>MALALWVFGLLDLICLASANIFEYQVDAQPLRPCELQRERAFLKREDYVPQCAEDGSFQTVQCGKDGASCWCVDADGREVPGSRQPGRPAACLSFCQLQKQQILLSSYINSTATSYLPQCQDSGDYSPVQCDLRRRQCWCVDAEGMEVYGTRQQGRPARCPRSCEIRNRRLLHGVGDRSPPQCSPDGAFRPVQCKFVNTTDMMIFDLVHSYSRFPDAFVTFSSFRSRFPEVSGYCYCADSQGRELAETGLELLLDEIYDTIFAGLDLASTFAETTLYRILQRRFLAVQLVISGRFRCPTKCEVERFAATSFRHPYVPSCHPDGEYQAAQCQQGGPCWCVDSRGQEIPGTRQRGEPPSCAEDQSCPSERRRAFSRLRFGPSGYFSRRSLLLAPEEGPVSQRFARFTASCPPSIKELFLDSGIFQPMLQGRDTRFVAPESLKEAIRGLFPSRELARLALQFTTNAKRLQQNLFGGRFLVKVGQFNLSGALGTRGTFNFSHFFQQLGLPGFQDGRALADLAKPLSVGLNSNPASEAPKASKIDVALRKPVVGSFGFEVNLQENQNALQFLSSFLELPEFLLFLQHAISVPEDIARDLGDVMEMVFSSQGCGQAPGSLFVPACTAEGSYEEVQCFAGDCWCVDAQGRELAGSRVRGGRPRCPTECEKQRARMQSLLGSQPAGSSLFVPACTSKGNFLPVQCFNSECYCVDTEGQPIPGTRSALGEPKKCPSPCQLQAERAFLGTVRTLVSNPSTLPALSSIYIPQCSASGQWSPVQCDGPPEQAFEWYERWEAQNSAGQALTPAELLMKIMSYREAASRNFRLFIQNLYEAGQQGIFPGLARYSSFQDVPVSVLEGNQTQPGGNVFLEPYLFWQILNGQLDRYPGPYSDFSAPLAHFDLRSCWCVDEAGQKLEGTRNEPNKVPACPGSCEEVKLRVLQFIREAEEIVTYSNSSRFPLGESFLAAKGIRLTDEELAFPPLSPSRETFLEKFLSGSDYAIRLAAQSTFDFYQRRLVTLAESPRAPSPVWSSAYLPQCDAFGGWEPVQCHAATGHCWCVDGKGEYVPTSLTARSRQIPQCPTSCERLRASGLLSSWKQAGVQAEPSPKDLFIPTCLETGEFARLQASEAGTWCVDPASGEGVPPGTNSSAQCPSLCEVLQSGVPSRRTSPGYSPACRAEDGGFSPVQCDPAQGSCWCVLGSGEEVPGTRVAGSQPACESPQCPLPFSVADVAGGAILCERASGLGAAAGQRCQLRCSQGYRSAFPPEPLLCSVQRRRWESRPPQPRACQRPQFWQTLQTQAQFQLLLPLGKVCSADYSGLLLAFQVFLLDELTARGFCQIQVKTAGTPVSIPVCDDSSVKVECLSRERLGVNITWKLQLVDAPPASLPDLQDVEEALAGKYLAGRFADLIQSGTFQLHLDSKTFSADTSIRFLQGDRFGTSPRTQFGCLEGFGRVVAASDASQDALGCVKCPEGSYFQDEQCIPCPAGFYQEQAGSLACVPCPEGRTTVYAGAFSQTHCVTDCQKNEVGLQCDQDSQYRASQRDRTSGKAFCVDGEGRRLPWTEAEAPLVDAQCLVMRKFEKLPESKVIFSADVAVMVRSEVPGSESSLMQCLADCALDEACGF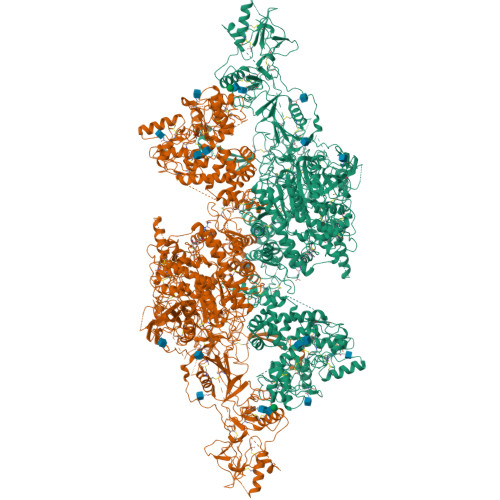LTVSTAGSEVSCDFYAWASDSIACTTSGRSEDALGTSQATSFGSLQCQVKVRSREGDPLAVYLKKGQEFTITGQKRFEQTGFQSALSGMYSPVTFSASGASLAEVHLFCLLACDHDSCCDGFILVQVQGGPLLCGLLSSPDVLLCHVRDWRDPAEAQANASCPGVTYDQDSRQVTLRLGGQEIRGLTPLEGTQDTLTSFQQVYLWKDSDMGSRSESMGCRRDTEPRPASPSETDLTTGLFSPVDLIQVIVDGNVSLPSQQHWLFKHLFSLQQANLWCLSRCAGEPSFCQLAEVTDSEPLYFTCTLYPEAQVCDDILESSPKGCRLILPRRPSALYRKKVVLQDRVKNFYNRLPFQKLTGISIRNKVPMSDKSISSGFFECERLCDMDPCCTGFGFLNVSQLKGGEVTCLTLNSLGLQTCSEEYGGVWRILDCGSPDTEVRTYPFGWYQKPVSPSDAPSFCPSVALPALTENVALDSWQSLALSSVIVDPSIRNFDVAHISTAAVGNFSAARDRCLWECSRHQDCLVTTLQTQPGAVRCMFYADTQSCTHSLQAQNCRLLLHEEATYIYRKPNIPLPGFGTSSPSVPIATHGQLLGRSQAIQVGTSWKPVDQFLGVPYAAPPLGEKRFRAPEHLNWTGSWEATKPRARCWQPGIRTPTPPGVSEDCLYLNVFVPQNMAPNASVLVFFHNAAEGKGSGDRPAVDGSFLAAVGNLIVVTASYRTGIFGFLSSGSSELSGNWGLLDQVVALTWVQTHIQAFGGDPRRVTLAADRGGADIASIHLVTTRAANSRLFRRAVLMGGSALSPAAVIRPERARQQAAALAKEVGCPSSSVQEMVSCLRQEPARILNDAQTKLLAVSGPFHYWGPVVDGQYLRETPARVLQRAPRVKVDLLIGSSQDDGLINRAKAVKQFEESQGRTSSKTAFSQALQNSLGGEAADAGVQAAATWYYSLEHDSDDXASFSRALEQATRDYFIICPVIDMASHWARTVRGNVFMYHAPESYSHSSLELLTDVLYAFGLPFYPAYEGQFTLEEKSLSLKIMQYFSNFIRSGNPNYPHEFSRRAPEFAAPWPDFVPRDGAESYKELSVLLPNRQGLKKADCSFWSKYIQSLKASADETKDGPSADSEEEDQPAGSGLTEDLLGLPELASKTYSK[2x]> XMEITNV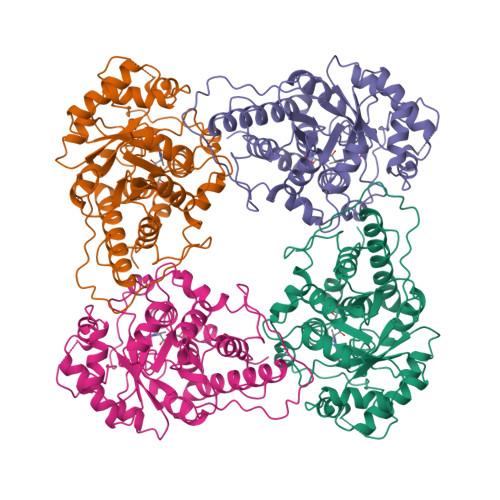NEYEAIAKQKLPKMVYDYYASGAEDQWTLAENRNAFSRILFRPRILIDVTNIDMTTTILGFKISMPIMIAPTAMQKMAHPEGEYATARAASAAGTIMTLSSWATSSVEEVASTGPGIRFFQLYVYKDRNVVAQLVRRAERAGFKAIALTVDTPRLGRREADIKNRFVLPPFLTLKNFEGIDLGKMDKANDSGLSSYVAGQIDRSLSWKDVAWLQTITSLPILVKGVITAEDARLAVQHGAAGIIVSNHGARQLDYVPATIMALEEVVKAAQGRIPVFLDGGVRRGTDVFKALALGAAGVFIGRPVVFSLAAEGEAGVKKVLQMMRDEFELTMALSGCRSLKEISRSHIAADWDGPSSRAVARL> VVKQDLSDNQYIQKKPNEITSNELLLPLPNDKLLGDPKAPILMIEYASLTCYHCSLFHRNVFP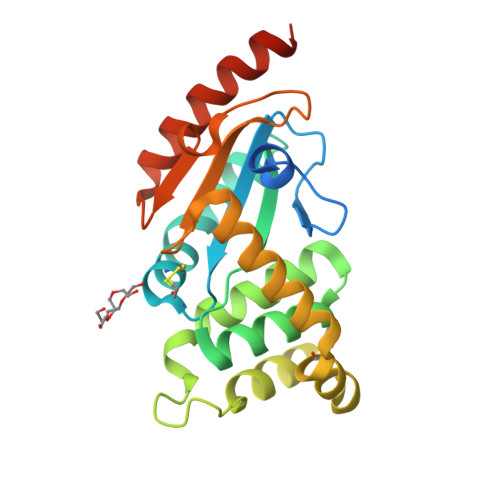KIKEKYIDTGKMLYIFRHFPLDYRGLKAAMLSHCYEKQEDYFNFNKAVFNSIDSWNYYNLSDLTLLQRIAALSNLKQDAFNQCINDKKIMDKIVNDKSLAINKLGITAVPIFFIKLNDDKSYIEHNKVKHGGYKELKYFTNVIDKLYGKAIVKLEHHHHHHHH>GSHMRTIIALETHDVRFPTSRELDGSDAMNPDPDYSAAYVVLRTDGAEDLAGYGLVFTIGRGNDVQTAAVAALAEHVVGLSVDKVIADLGAFARRLTNDSQLRWLGPEKGVMHMAIGAVINAAWDLAARAANKPLWRFIAELTPEQLVDTIDFRYLSDALTRDEALAILRDAQPQRAARTATLIEQGYPAYTTSPGWLGYSDEKLVRLAKEAVADGFRTIKLKVGANVQDDIRRCRLARAAIGPDIAMAVDANQRWDVGPAIDWMRQLAEFDIAWIEEPTSPDDVLGHAAIRQGITPVPVSTGEHTQN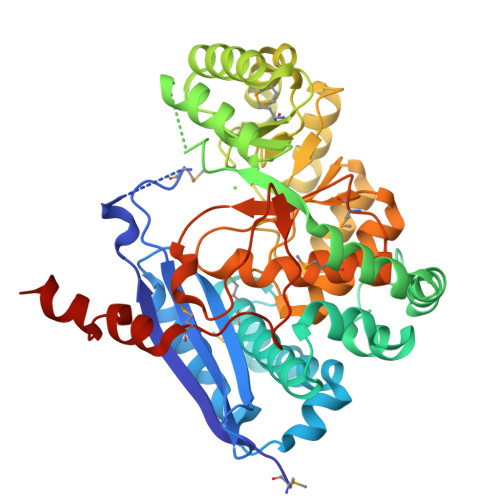RVVFKQLLQAGAVDLIQIDAARVGGVNENLAILLLAAKFGVRVFPHAGGVGLCELVQHLAMADFVAITGKMEDRAIEFVDHLHQHFLDPVRIQHGRYLAPEVPGFSAEMHPASIAEFSYPDGRFWVEDLAASKAKA[4x]> MRTFDLEEKLQTNKYNANFVTFMEGKDFNVEYIQRGGLRDPLIFKNSDGLGIKMPDPDFTVNDVKMCVGSRRMVDVMDVNTQKGIEMTMAQWTRYYETPEEEREKLYNVISLEFSHTRLENMVQRPSTVDFIDWVDNMWPRHLKESQTESTNAILEMQYPKVQKYCLMSVRGCYTDFHVDFGGTSVWYHIHQGGKVFWLIPPTAHNLELYENWLLSGKQGDIFLGDRVSDCQRIELKQGYTFVIPSGWIHAVYTPTDTLVFGGNF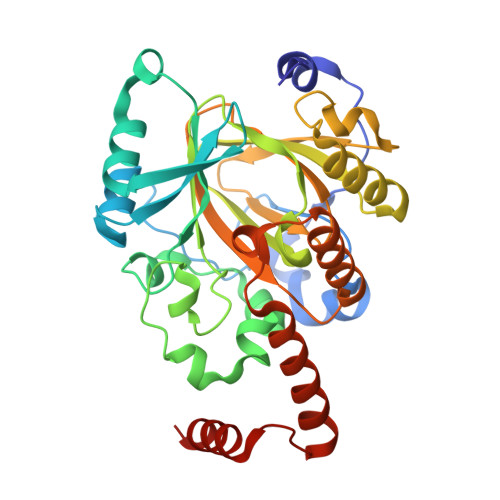LHSFNIPMQLKIYSIEDRTRVPNKFRYPFYYEMCWYVLERYVYCITNRSHLTKDFQKESLSMDME>[3x]GSSGSSGMTQLALIGLWIGFIGMVIGAVIFGQKAVAMRRKEGMEFPLKSFFIVLWAGALYLTMILGETVTPVKDQTVFWGRYVDWVVTTPVLLLDLGVLAGLRPKLIAGVIAADIFMILTGLVATLEAPPTSYLWYIISCGAFIAILASLLTEFTASAARRNVRVNNLFLKLRNYLIVLWICYPIVWL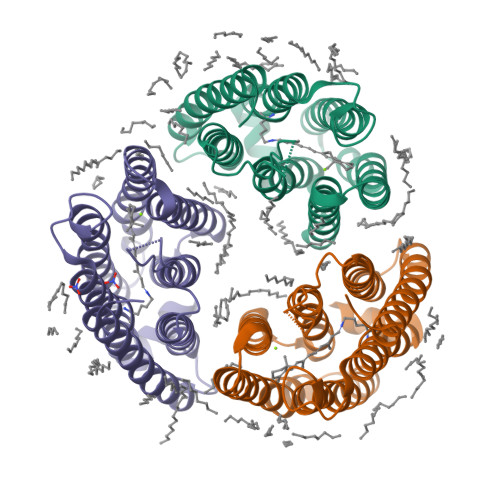LGAEAFKIIPTGVEVVIYAIIDIAAKVGFGLILTSAAPEILAQASNSESFMEAVHSYMGKGERERDRSYTP>[2x]MYKTLRLGDRGADVSYLQRQLIAAGARLDIDAIYGSATRDAVMAFQATHGLVADGIAGPKTWSTLSAGRRDPRHLTDADLQRAADRLQVDLAAVRAVNEVESKGAGFLPDGRPVILYERHIMYRQLAAAGLDADALAAKYPALVNSKRGG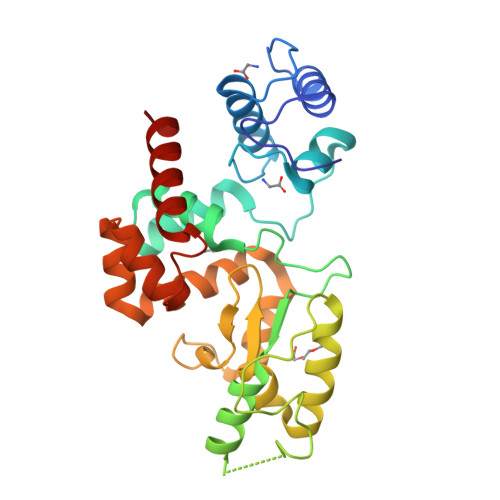YAGDAAEYARLASASQISGACALEATSWGAFQIMGFHWKALGYPDVFAFVDAMKVSEAEQLEAFVRFVLADKVMLAALRSKKWAKFAELYNGKAYAENLYDVKLERAFDRYSRAAA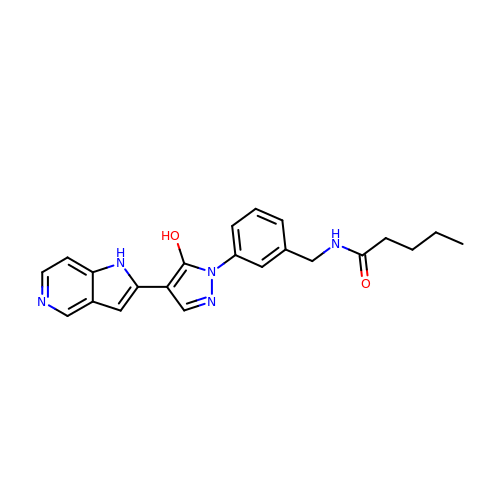N-({3-[5-hydroxy-4-(1H-pyrrolo[3,2-c]pyridin-2-yl)-1H-pyrazol-1-yl]phenyl}methyl)pentanamide | C22 H23 N5 O2 | QHVJCCLHYRIBOU-UHFFFAOYSA-N>[24x]LLKEYKNAWDKYDDKQLKEVFAL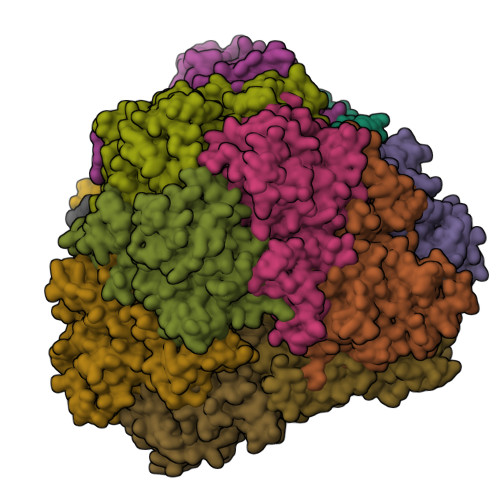GDRFKNFISNCKTERECVTELIKTAEKSGYRNIEDILAKGETLKEGDKVYANNRGKGLIMFLIGKEPLYTGFKILGAHIDSPRLDLKQNPLYEDTDLAMLETHYYGGIKKYQWVTLPLAIHGVIVKKDGTIVNVCVGEDDNDPVFGVSDILVHLASEQLEKKASKVIEGEDLNILIGSIPLKDGEEKQKVKHNIMKILNEKYDISEEDFVSAELEIVPAGKARDYGFDRSMVMGYGQDDRICAYTSFEAMLEMKNAKKTCITILVDKEEVGSIGATGMQSKFFENTVADIMSLCGDYDELKLRKALYNSEMLSSDVSAAFDPNYPNVMEKRNSAYLGKGIVFNKYTGSRGKSGCNDANPEYIAELRRILSKESVNWQTAELGKVDQGGGGTIAYILAEYGMQVIDCGVALLNMHAPWEISSKADIYETKNGYSAFLNN>[3x]FSSREQPQQNEGQIQKLNALKPDNRIESEGGLIETWNPNNKPFQCAGVALSRCTLNRNALRRPSYTNGPQEIYIQQGKGIFGMIYPGCPSTFEEPQQPQQRGQSSRPQDRHQKIYNFREGDLIAVPTGVAWWMYNNEDTPVVAVS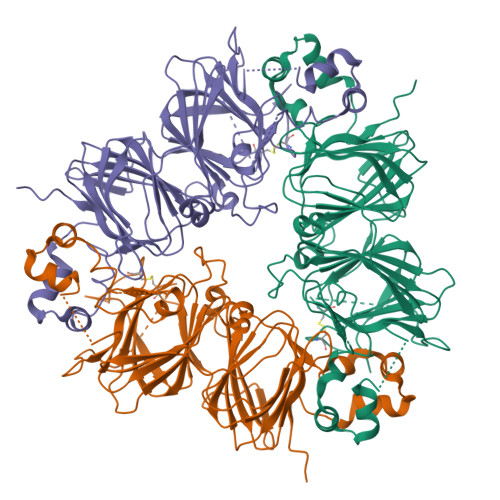IIDTNSLENQLDQMPRRFYLAGNQEQEFLKYQQEQGGHQSQKGKHQQEEENEGGSILSGFTLEFLEHAFSVDKQIAKNLQGENEGEDKGAIVTVKGGLSVIKPPTDEQQQRPQEEEEEEEDEKPQCKGKDKHCQRPRGSQSKSRRNGIDETICTMRLRHNIGQTSSPDIYNPQAGSVTTATSLDFPALSWLRLSAEFGSLRKNAMFVPHYNLNANSIIYALNGRALIQVVNCNGERVFDGELQEGRVLIVPQNFVVAARSQSDNFEYVSFKTNDTPMIGTLAGANSLLNALPEEVIQHTFNLKSQQARQIKNNNPFKFLVPPQESQKRAVA4-[(3S)-3-{[(2E)-but-2-enoyl]amino}piperidin-1-yl]-5-fluoro-2,3-dimethyl-1H-indole-7-carboxamide | C20 H25 F N4 O2 | 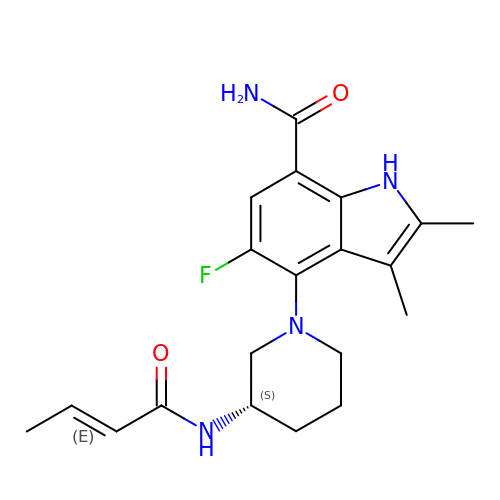BCSXUDNOTSZTNK-BPJJOFIESA-N>[3x]GPGYQDPGNIQIQSMPKVKERVSVPSKDDTIYSYHDSIKDSIKAVVNISTEKKIKNNFIGGGVFNDPFFQQFFGD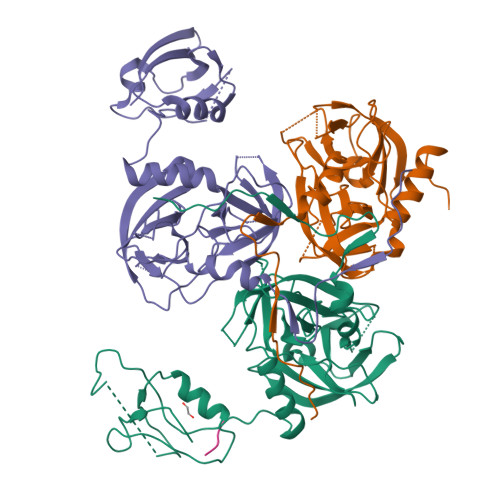LGGMIPKERMERALGSGVIISKDGYIVTNNHVIDGADKIKVTIPGSNKEYSATLVGTDSESDLAVIRITKDNLPTIKFSDSNDISVGDLVFAIGNPFGVGESVTQGIVSALNKSGIGINSYENFIQTDASINPGNSGGALIDSRGGLVGINTAIISKTGGNHGIGFAIPSNMVKDTVTQLIKTGKIERGYLGVGLQDLSGDLQNSYDNKEGAVVISVEKDSPAKKAGILVWDLITEVNGKKVKNTNELRNLIGSMLPNQRVTLKVIRDKKERAFTLTLAERK;> AAAA> VHHPPSYVAHLASDFGVRVFQQVAQASKDRNVVFSPYGVASVLAMLQLTTGGETQQQIQAAMGFKIDDKGMAPALRHLYKELMGPWNKDEISTTDAIFVQRDLKLVQGFMPHFFRLFRSTVKQVDFSEVERARFIINDWVKTHTKGMISNLLGKGAVDQLTRLVLVNALYFNGQWKTPFPDSSTHRRLFHKSDGSTVSVPMMAQTNKFNYTEFTTPDGHYYDILELPYHGDTLSMFIAAPYEKEVPLSALTNILSAQLISHWKGNMTRLPRLLVLPKFSLETE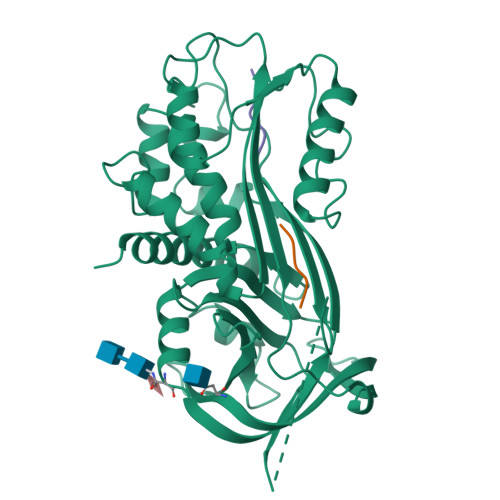VDLRKPLENLGMTDMFRQFQADFTSLSDQEPLHVAQALQKVKIEVNESGTVESSSTAVIVSARMAPEEIIMDRPFLFVVRHNPTGTVLFMGQVMEP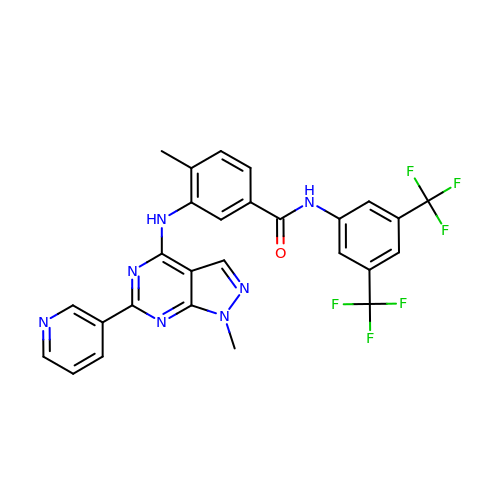~{N}-[3,5-bis(trifluoromethyl)phenyl]-4-methyl-3-[(1-methyl-6-pyridin-3-yl-pyrazolo[3,4-d]pyrimidin-4-yl)amino]benzamide | C27 H19 F6 N7 O | VIKHFAMUADDHTH-UHFFFAOYSA-N> GSAEYVRALFDFNGNDEEDLPFK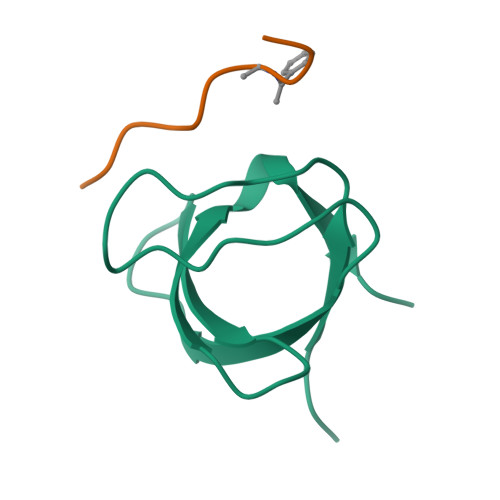KGDILRIRDKPEEQWWNAEDSEGKRGMIPVPYVEKYHHHHHH;> YEVPGPVPPRRR(3S)-1-[(3-phenyl-1,2,4-oxadiazol-5-yl)methyl]pyrrolidin-3-ol 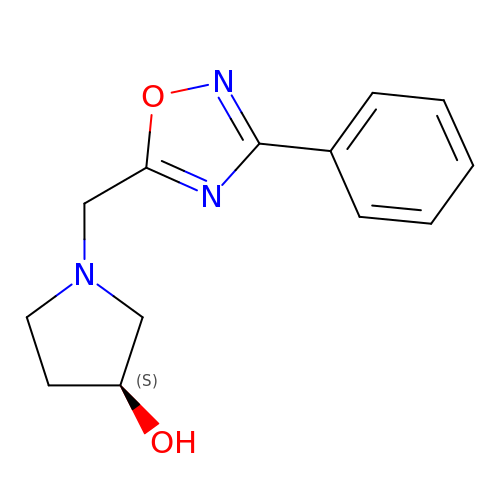| C13 H15 N3 O2 | FQHRNVUXCKTULP-NSHDSACASA-N INOSINE 5'-TRIPHOSPHATE | C10 H15 N4 O14 P3 | 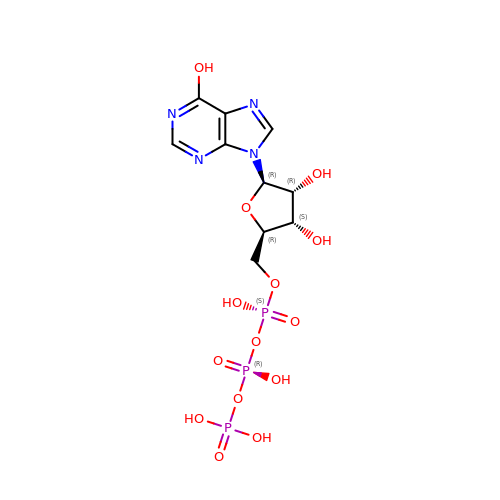HAEJPQIATWHALX-KQYNXXCUSA-N>[2x]SNAMRKLNNHDVHKRYQDRLEEDVEFTINYELPLSCLWSTIKDFSSDFEEKTEAFFILFKELLRRGHLKLQRDGQIIGHTPEEWEQIFREVWPE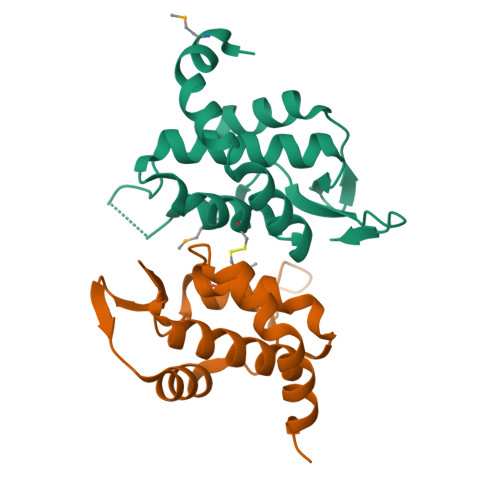YEIEPNPLPGYAPFDIGMWLTVEAPAYAVWIDPEDGSEYWAG>[4x]GRKERERLEEKLEDANERIAELVKLEERQRIARDLEDTLGQKLSLIGLKSDLARKLIYKDPEQAARELKSVQQTARTSLNEVRKIVSSMKGIRLKDELINIKQI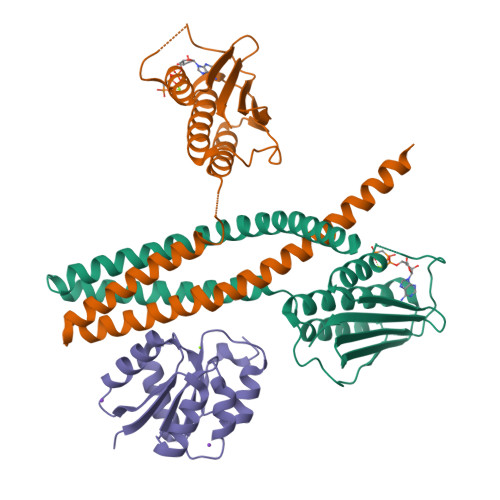LEAADIMFIYEEEKWPENISLLNENILSMCLKEAVTNVVKHSQAKTCRVDIQQLWKEVVITVSDDGTFKGEENSFSKGHGLLGMRERLEFANGSLHIDTENGTKLTMAIPNNSK;>GSGSMISIFIAEDQQMLLGALGSLLNLEDDMEVVGKGTTGQDAVDFVKKRQPDVCIMDIEMPGKTGLEAAEELKDTGCKIIILTTFARPGYFQRAIKAGVKGYLLKDSPSEELANAIRSVMNGKRIYAPELMEDLYSEA[2x]> IGTGFPFDPHYVEVLGERMHYVDVGPRDGTPVLFLHGNPTSSYLWRNIIPHVAPSHRCIAPDLIGMGKSDKPDLDYFFDDHVRYLDAFIEALGLEEVVLVIHDWGSALGFHWAKRNPERVKGIACMEFIRPIPTWDEWPEFARELFQAFRTADVGRELIIDQNAFIEQVLPKFVVRPLTEVEMDHYREPFLKPVDREPLWRFPNELPIAGEPANIVALVEAYM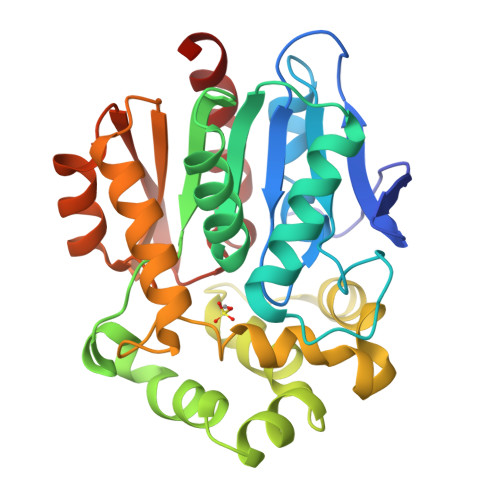NWLHQSPVPKLLFWGTPGVLIPPAEAARLAESLPNCKTVDIGPGLHYLQEDNPDLIGSEIARWLPAL>AMADLEQKVLEMEASTYDGVFIWKISDFARKRQEAVAGRIPAIFSPAFYTSRYGYKMCLRIYLNGDGTGRGTHLSLFFVVMKGPNDALLRWPFNQKVTLMLLDQNNREHVIDAFRPDVTSSSFQRPVNDMNIASGCPLFCPVSK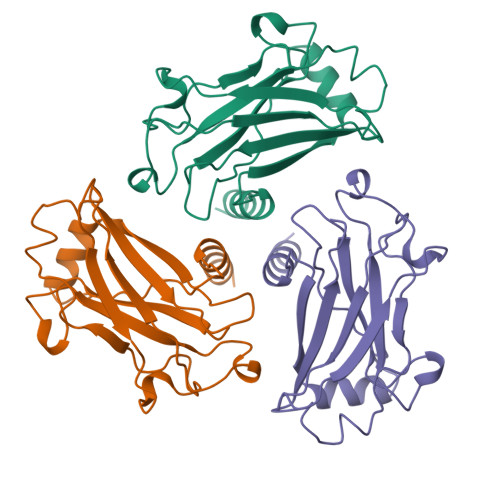MEAKNSYVRDDAIFIKAIVDLTGL[6x]The main replication protein NS1 plays a critical role in cell cycle arrest, transactivation of viral and host genes, and replication and package of B19V genome. Based on its similarity to other parvoviral replication proteins, such as Rep72 of the adeno-associated virus (AAV), NS1 is predicted to contain one nuclease domain (Nuc, aa 1–176), one oligomerization domain (OD, aa 201–270), one SF3 helicase domain (SF3 HD, aa 271–501), and one zinc-binding domain (ZnD, aa 571–671). The SF3 HD domain of NS1 belongs to the SF3 helicase superfamily, which unwinds DNA with 3′→5′ polarity. Totally, four cryo-electron microscopy (cryo-EM) structures were determined, which revealed the detailed mechanisms for ATP binding and hydrolysis and DNA binding and unwinding by NS1.

To reveal how NS1_2-570 assembles, we performed cryo-EM study and solved one NS1_2-570/AMPPNP binary complex. The NS1_2-570/AMPPNP complex was determined at an overall resolution of 2.75 Å. NS1_2-570 exists as a dodecamer in the structure. The dodecamer has a height of 120 Å and it is formed by two hexamers. Each hexamer adopts a double-layered ring-shaped conformation; the top and bottom layers are formed by the OD and SF3 HD domains, respectively. Since no density was observed for the residues within the 2–201, 279–285, and 500–570 regions, they were not modeled in the final structure. In the NS1_2-570/AMPPNP complex, one AMPPNP molecule is captured at the characteristic Walker A region of each NS1 protomer. The α- and β-phosphate groups of AMPPNP form H-bond interactions with the main chains of Ser331, Lys334, and Asn336. The γ-phosphate H-bonds with the side chain of Lys334. Both β- and γ-phosphate groups coordinate with an Mg2+ cation, which is six-coordinated. In contrast, the ATP-binding pocket is widely open in the NS1_2-570/AMPPNP complex.

>[12x]ELFRGVLQVSSNVLDCANDNWWCSLLDLDTSDWEPLTHTNRLMAIYLSSVASKLDFTGGPLAGCLYFFQVECNKFEEGYHIHVVIGGPGLNPRNLTVCVEGLFNNVLYHLVTGNVKLKFLPGMTTKGKYFRDGEQFIENYLMKKIPLNVVWCVTNIDGYIDTCISATFRRGACHAKKPRMTTAINDTSSDAGEPSGTGAEVVPFNGKGTKASIKFQTMVNWLCENRVFTEDKWKLVDFNQYTLLSSSHSGSFQIQSALKLAIYKATNLVPTSTFLLHADFEQVMCIKDNKIVKLLLCQNYDPLLVGQHVLKWIDKKCGKKNTLWFYGPPSTGKTNLAMAIAKSVPVYGMVNWNNENFPFNDVAGKSLVVWDEGIIKSTIVEAAKAILGGQPTRVDQKMRGSVAVPGVPVVITSNGDITFVVSGNTTTTVHAKALKERMVKLNFTVRCSPDMGLLTEADVQQWLTWCNAQSWDHYENWAINYTFDFPGINADALHPDLQTTPIVTDTSISSSGGESSEELSESSFFNLITPGACNTETPRSSTPIPGTSSGESLVGSPVSSEVVAASWEE> QQQTLPKPFIWAEPHFMVPKEKQVTICCQGNYGAVEYQLHFEGSLFAVDRPKPPERINKVKFYIPDMNSRMAGQYSCIYRVGELWSEPSNLLDLVVTEMYDTPTLSVHPGPEVISGEKVTFYCRLDTATSMFLLLKEGRSSHVQRGYGKVQAEFPLGPVTTAHRGTYRCFGSYNNHAWSFPSEPVKLLVTGDIENTSLAPEDPTFPADTWGTYLLTT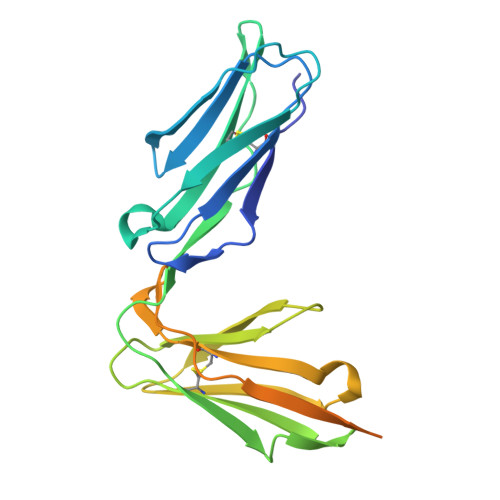ETGLQKDHALWDHTAQNLLRMGLAF> KPKLLNKFDKTIKAELDAAEKLRKRGKIEEAVNAFKELVRKYPQSPRARYGKAQCEDDLAEKRRSNEVLRGAIETYQEVASLPDVPADLLKLSLKRRSDRQQFLGHMRGSLLTLQRLVQLFPNDTSLKNDLGVGYLLIGDNDNAKKVYEEVLSVTPNDGFAKVHYGFILKAQNKIAESIPYLKEGIESGDPGTDDGRFYFHLGDAMQRVGNKEAYKWYELGHKRGHFASVWQRSLYNVNGLKAQPWWTPKETGYTELVKSLERNWKLIRDEGLAVMDKAKGLFLPEDENLREKGDWSQFTLWQQGRRNENACKGAPKTCTLLEKFPETTGCRRGQIKYSIMHPGTHVWPHTGPTNCRLRMHLGLVIPKEGCKIRCANETKTWEEGKVLIFDDSFEHEVWQDASSFRLIFIVDVWHPELTPQQR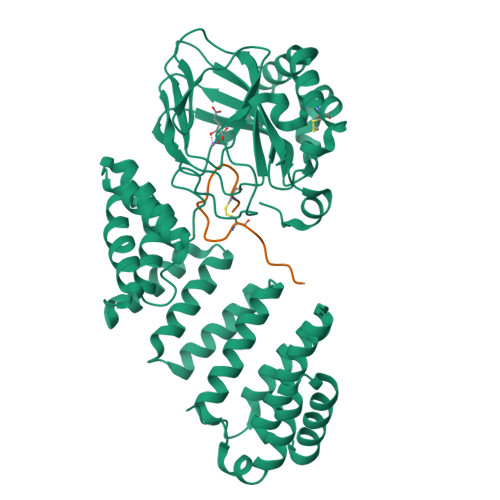RSLPAI;> DGDQSETSPSQNQGKCKDGLGEYTCTSLEGFEGKNSELF> ATIAALLSA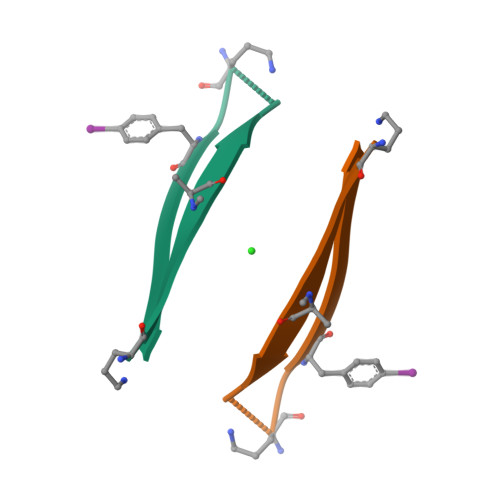SFSTTAV> GMMNTTQEGRQRL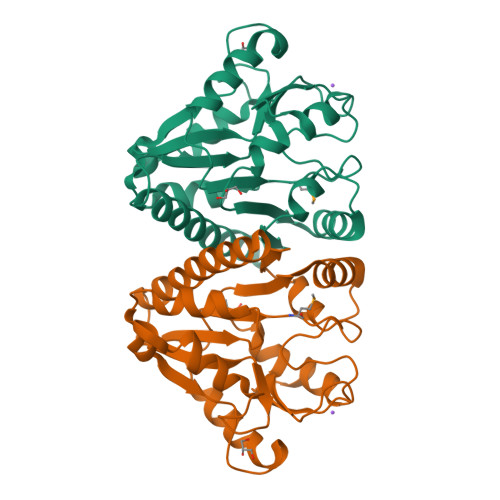AERLADTVAQALEADLAKRERALLVVSGGSTPKPFFTSLAAKALPWARVDVTLADERWVTADDADSNARLVRETLLVGPAAEACFHPLTTDDDTPEAGVETVAERLESLPWPASAVILGMGGDGHTASLFPDSEQLATALETTSAAVVVHAPSVPQARITLSASRLADAGLHVLHITGNDKRRVLAEALAGDDVRQLPIRAFLSQPIATYWAP The UNC-45 chaperone controls myosin function mediating the folding, assembly, and degradation of the muscle protein. UNC-45, which is present in all eukaryotes, employs a UCS domain to interact with myosin, a central domain that mediates oligomerization, and a TPR domain that interacts with members of the protein quality control (PQC) network. In addition to functioning as a folding factor of the myosin motor, UNC-45 can form linear protein chains that provide regular spaced docking sites for HSP70 and HSP90. Structural analysis of a minimal chaperone:substrate complex reveals that UNC-45 binds to a conserved FX3HY motif in the myosin motor domain.

Given the difficulties in obtaining a co-crystal structure with C. elegans UNC-45, we moved to the less complex fungal orthologue SHE4. Despite lacking the TPR-domain, SHE4 contains a functional UCS-domain for myosin binding. Isothermal titration calorimetry (ITC) measurements showed that 13 residues (561–573) comprise the core of the myosin motif, binding to SHE4KL with a KD of 0.6 μM. After intense co-crystallization trials with various myosin peptides, we obtained a well-diffracting SHE4 co-crystal with a peptide comprising Myo4 residues 561–581. We determined the co-crystal structure at a resolution of 2.4 Å and were able to visualize a minimal SHE4:Myo4 complex in atomic detail. In this structure, the Myo4 residues Lys561-Phe562-Ile563-Val564-Ser565-His566-Tyr567 were well-defined by electron density. The eight myosin residues are accommodated in the UCS-canyon by a dense network of hydrogen bonds and hydrophobic interactions. The tight binding mode forces the Myo4 peptide to adopt a bent conformation, with its C-terminal portion being directed out of the central groove of the UCS-domain. ITC-measurements showed that binding to the myosin peptide was abrogated in the N475A mutant, confirming its participation in substrate binding. Taken together, our structural and biochemical data indicate that the conserved myosin residues Phe577, His581 and Tyr582 mediate binding to C. elegans UNC-45. We propose that the conserved FX3HY motif represents a universal and highly specific substrate epitope, recognized by the myosin-specific chaperone UNC-45.

> MNKVWDRIVGSDSADAQSVLKERCSSPKDVTDLLHVIQNWTSEIHNNGEETRCWKCVPMLAGYVKDWGQLEFLCRRILLRSSIQEIRPLLLVTMKSLMSNHSDNTEQKCGNILQQLLIEAEEDSGNVSLRLLVDAMSLVFPICLGVCRDMFLSTDFQDILTRNLNSSADDEHLVNGALRLLAVSCIDEAVRRFIAEHYLKTLQQSFKVEKYKVLTALVLIKIWSFTKIEKETLNSCINLFIDSLSNGENIEINTEALAYLTLKPSVRVLLRGNGDVCLKIIELIKSQDTTPTDLYGLLIILANVSEHPSQNEDTVDKLKASLKTNQEKNDEPTLENVKDIEEFNRDYIIDLDLIGSLKSIKLSTSSYNQAIRIIYNVTRDKTQISECVKQGAGLMLLVFLAQKRNLSKDEWYLLSIRALSKTLIYVNPETAFSKYSPLSAAPFLFENLPLPNDNALSELQFTQLDTYEALLALTNLATINQGVDLGKIILSNAQYWDSIENLLLDSSVRIQRSTLELISNLMSNPMAISAKFFCFENPKSAQNFEILVKLLELHDIQSQRAVAAIFANIASTVPFICKELSEKRNLIETAIRVFKTQNTDTDLRIRLLVLLSSIFNANAHAVACVKNDEEFVKELQKYRNTPSQKDPLTPELSKEILSLINLEHHHHHH;> KFIVSHY> MMTKVDFWPTLKDAYEPLYPQQLEILRQQVVS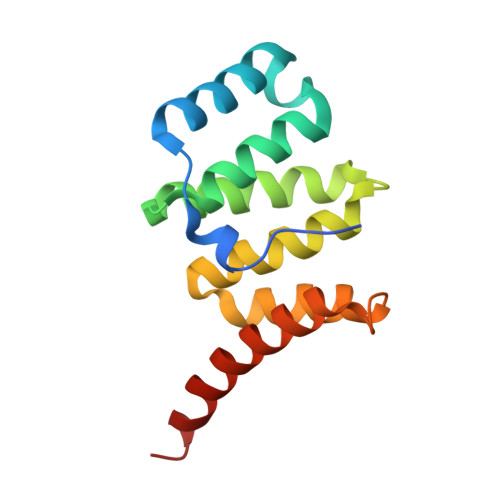EGGPTATIQSRFNYAWGLIKSTDVNDERLGVKILTDIYKEAESRRRECLYYLTIGCYKLGEYSMAKRYVDTLFEHERNNKQVGALKSMVEDKIQKEENLYFQ> EPQTTLHKTITPISGQDDKYELSL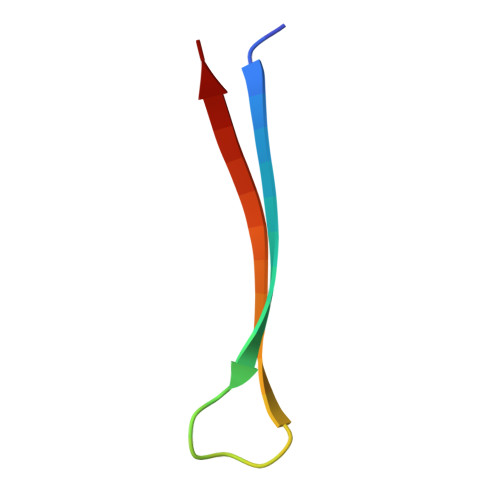DITSKL>MEKQQDLPFPYEFRELNPEEDKLVKANLGAFPTTYVKLGPKGYMVYRPYL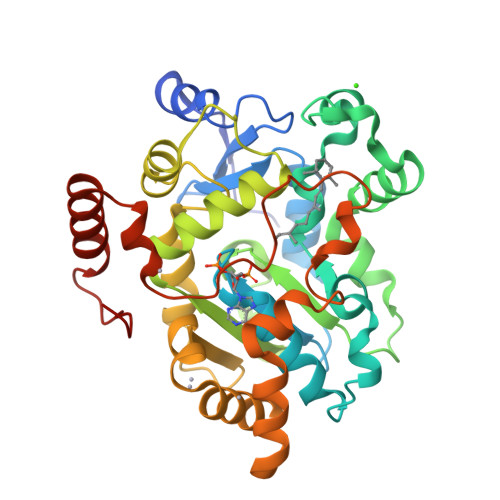KDAANIYNMPLRPTDVFVASYQRSGTTMTQELVWLIENDLNFEAAKTYMSLRYIYLDGFMIYDPEKQEEYNDILPNPENLDMERYLGLLEYSSRPGSSLLAAVPPTEKRFVKTHLPLSLMPPNMLDTVKMVYLARDPRDVAVSSFHHARLLYLLNKQSNFKDFWEMFHRGLYTLTPYFEHVKEAWAKRHDPNMLFLFYEDYLKDLPGCIARIADFLGKKLSEEQIQRLCEHLNFEKFKNNGAVNMEDYREIGILADGEHFIRKGKAGCWRDYFDEEMTKQAEKWIKDNLKDTDLRYPNMEL[2x]One especially common junction element is the kink-turn (k-turn). k-turns are elements in double-stranded RNA that introduce a tight kink into the helical axis, with an included angle close to 50°. A standard k-turn comprises a three-nucleotide bulge followed by successive G•A and A•G trans G(sugar edge)•A(Hoogsteen edge) basepairs. k-turns are commonly-occurring motifs that introduce sharp kinks into duplex RNA, thereby facilitating tertiary contacts. Both the folding and conformation of k-turns are determined by their local sequence. k-turns fall into two conformational classes, called N3 and N1, that differ in the pattern of hydrogen bonding in the core. We show here that this is determined by the basepair adjacent to the critical G•A pairs.

We therefore decided to extend the study with a systematic structural analysis of HmKt-7 as a function of the 3b,3n sequence. This was performed in the constant environment of the SAM-I riboswitch, modified by replacing its natural k-turn by HmKt-7 with different 3b,3n sequences. In this way we could observe the effect of changing the 3b,3n sequence alone in an otherwise completely unchanged RNA molecule. Thus, there are three examples each of 3b,3n = G–C and U•U, all of which are k-turns that adopt the N3 conformation. Where the modified HmKt-7 elements have the same 3b,3n sequence as a different k-turn, they adopt the same conformation as that structure. The N3 group contain a preponderance of 3b,3n = A•G and U•U pairs, and the N1 group comprise mainly 3b,3n = U•G, C•A and C•C pairs. Moreover, the structures of the HmKt-7 variants inserted into the SAM-I riboswitch demonstrate that changing the 3b,3n sequence is sufficient to switch the equilibrium conformation of the k-turn.

> GGCUUAUCAAGAGAGGGUGAGCGACUGGCGCGAAGAUCCCCGGCAACCAGAAAUGGUGCCAAUUCCUGCAGCGGAAACGUUGAAAGAUGAGCC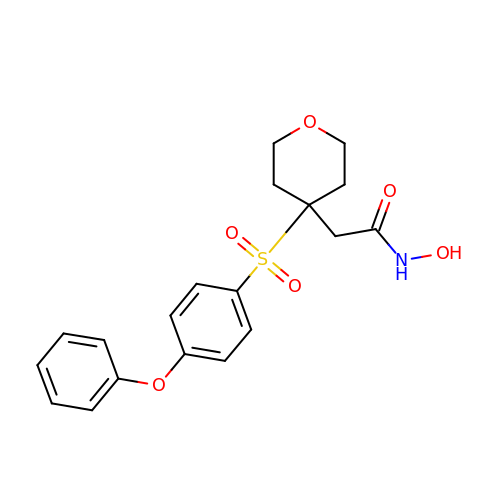N-HYDROXY-2-[4-(4-PHENOXY-BENZENESULFONYL)-TETRAHYDRO-PYRAN-4-YL]-ACETAMIDE | C19 H21 N O6 S | ARIRIZBKMKMEBD-UHFFFAOYSA-N>GPHMMSGEKRVLSGRVAVVTGSRKGIGLGIAMRLAMAG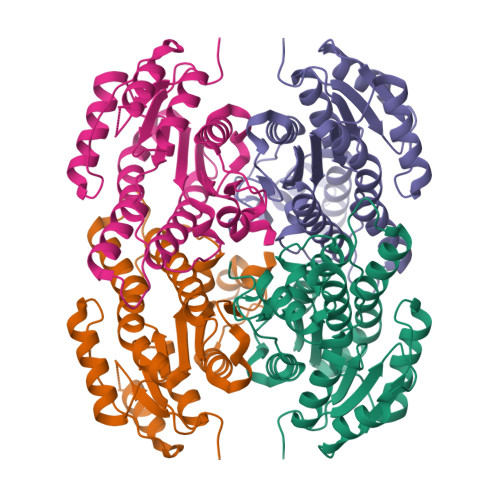ADVVLNGRRQSPEDSAIVEKVAAYGTRVRCFAANMKDRAQVEALIKFTEKELGAVEILVNNAGIQHVSPVETFPSDKWDEIIALNLTSAFHATQLCLPSMRQRGWGRIINIASVQGLVGSMNKSAYCAAKHGLIGFTKVVALETATTGITCNAICPGYVYTPLVEEQIKAVAEAKYGGDMEAATQAFLCEKQPAKAFVTVEQVGDAAVFLASPGADMIRGTTITVDGGWVAQ[2x]> GPHMLGILNKMFDPTKRTLNRYEKIANDIDAIRGDYENLSDDALKHKTIEFKERLEKGATTDDLLVEAFAVVREASRRVTGMFPFKVQLMGGVALHDGNIAEMKTGEGKTLTSTLPVYLNALTGKGVHVVTVNEYLASRDAEQMGKIFEFLGLTVGLNLNSMSKDEKREAYAADITYSTNNELGFDYLRDNMVLYKEQMVQRPLHFAVIDEVDSILIDEARTPLIISGQAAKSTKLYVQANAFVRTLKAEKDYTYDIKTKAVQLTEEGMTKAEKAFGIDNLFDVKHVALNHHINQALKAHVAMQKDVDYVVEDGQVVIVDSFTGRLMKGRRYSEGLHQAIEAKEGLEIQNESMTLATITFQNYFRMYEKLAGMTGTAKTEEEEFRNIYNMQVVTIPTNRPVVRDDRPDLIYRTMEGKFKAVAEDVAQRYMTGQPVLVGTVAVETSELISKLLKNKGIPHQVLNAKNHEREAQIIEEAGQKGAVTIA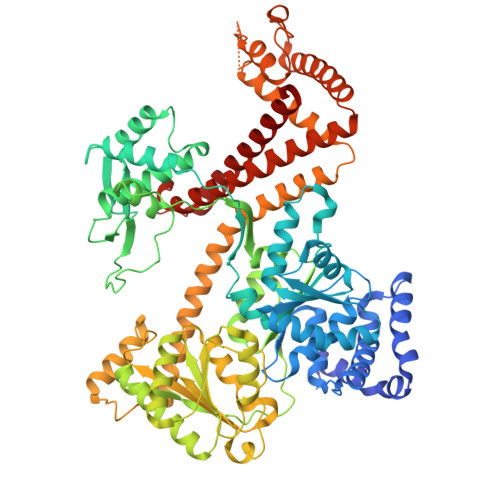TNMAGRGTDIKLGEGVKELGGLAVVGTERHESRRIDNQLRGRSGRQGDPGITQFYLSMEDELMRRFGAERTMAMLDRFGMDDSTPIQSKMVSRAVESSQKRVEGNNFDSRKQLLQYDDVLRQQREVIYKQRFEVIDSENLREIVENMIKSSLERAIAAYTPREELPEEWKLDGLVDLINTTYLDEGALEKSDIFGKEPDEMLELIMDRIITKYNEKEEQFGKEQMREFEKVIVLRAVDSKWMDHIDAMDQLRQGIHLRAYAQTNPLREYQMEGFAMFEHMIESIEDEVAKFVMKAEI> MVPISPIETVPVKLKPGMDGPKVKQWPLTEEKIKALVEICTEMEKEGKISKIGPENPYNTPVFAIKKKDSTKWRKLVDFRELNKRTQDFWEVQLGIPHPAGLKKKKSVTVLDVGDAYFSVPLDEDFRKYTAFTIPSINNETPGIRYQYNVLPQGWKGSPAIFQSSMTKILEPFKKQNPDIVIYQYMDDLYVGSDLEIGQHRTKIEELRQHLLRWGLTTPDKKHQKEPPFLWMGYELHPDKWTVQPIVLPEKDSWTVNDICKLVGKLNWASQIYPGIKVRQLSKLLRGTKALTEVIPLTEEAELELAENREILKEPVHGVYYDPSKDLIAEIQKQGQGQWTYQIYQEPFKNLKTGKYARMRGAHTNDVKQLTEAVQKITTESIVIWGKTPKFKLPIQKETWETWWTEYWQATWIPEWEFVNTPPLVKLWYQLEKEPIVGAETFYVDGAANRETKLGKAGYVTNKGRQKV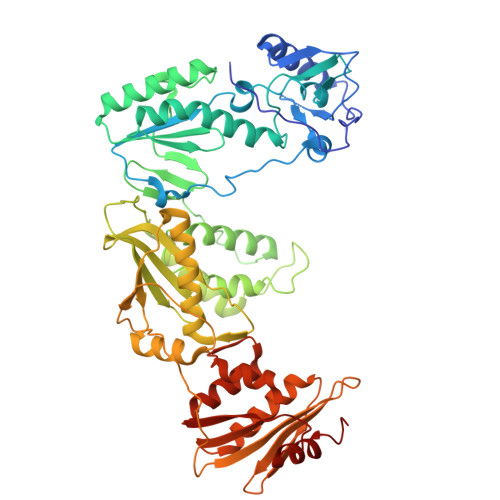VPLTNTTNQKTQLQAIYLALQDSGLEVNIVTDSQYALGIIQAQPDKSESELVNQIIEQLIKKEKVYLAWVPAHKGIGGNEQVDKLVSAGIRKIL>[3x]MASINLPFSLSGSKRIPTSEELADGYQCGPLDVELDNWLMWWLTGQVDGVIEGAGLTTDDTDLARL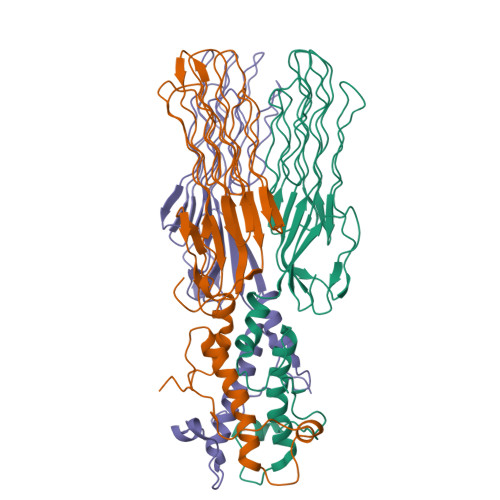YKAIQSMTSGNLRTVVLTAASGNLPIPSDVSVLNWVRAVGGGGAGGNSNTGNSKASGGGGGAGFDRFNVAVTPGSNVPYTVGAAGAVNGLGAGYNGGAGGSTAILGTTAGGGAGGLGVNNNATAVQVNGGTTSGTTPEISYPGGLGTEGIVGTGGGSVLSQPTQRAFTNAGNNNPANSWGGGGPGGSDFGGAWQPGGVGKQGIIIVQYFSRFAP>[2x]GFDYDVVVVGGGFAGATAARECGLQGYRTLLLEARSRLGGRTFTSRFAGQEIELGGTWVHWLQPHVWAEMQRYGLGVVEDPLTNLDKTLIMYNDGIVESISPDEFGKNIRIAFEKLCHDAWEVFPRPHEPMFTERARELDKSSVLDRIKTLGLSRLQQAQINSYMALYAGETTDKFGLPGVLKLFACGGWNYDAFMDTETHYRIQGGTIGLINAMLTDSGAEVRMSVPVTAVEQVNGGVKIKTDDDEIITAGVVVMTVPLNTYKHIDFTPALSKGKQRFIKEGQLSKGAKLYVHVKQNLGRVFAFADEQQPLNWVQTRDYSDELGTILSITIARKETIDVNDRDAVTREVQKMFPGVEVLGTAAYDWTADPFSLGAWAAYGVGQLSRLKDLQAAEGRIVFAGAETSNGWHASIDGAVESGLRAGREVKQLLS

Nicotine oxidoreductase (NicA2) is a flavin-dependent enzyme that catalyzes the degradation of nicotine into the non-psychoactive metabolite N-methylmyosmine (NMM). NicA2 acts by degrading nicotine in the bloodstream before it reaches the brain. Clinical use of NicA2 is limited by its poor catalytic activity in the absence of its natural electron acceptor CycN. The higher in vivo activity of NicA2 is due to the presence of a cytochrome c, termed CycN, that acts as an alternative electron acceptor to O29.

We were unable to solve structures of NicA2 v320 but were fortunate to obtain well-diffracting crystals of NicA2 v321 in both the ligand-free and NMM-bound forms. By contrast, the NMM-bound structures of v321 and wild-type NicA2 are very similar with an overall root mean squared deviation of <0.5 Å and no obvious difference that would explain our observed change in activity with O2. Our stopped-flow experiments demonstrated that NicA2 v321 has an increased rate of oxidation compared to the wild-type enzyme, but only when it is bound by the reaction product NMM. The observed increase in the oxidation rate of NMM-bound NicA2 v321 raises an intriguing possibility that the mutations in this variant alter the transport pathway of O2. After addition of NMM to NicA2 v321, we observed a substantial downfield chemical shift in the major peak of the enzyme, possibly due to conformational rearrangement in the tunnel region. We confirmed that these conformational changes are relevant to catalysis by observing a similar spectrum after the addition of nicotine to the enzyme to achieve the NMM-bound, reduced enzyme state that was rapidly oxidized by O2 in our kinetic experiments. Therefore, observations made using the NMM-bound oxidized enzyme report on the conformation of the enzyme relevant for the oxidation step. After NMM binding, NicA2 v321 undergoes major rearrangements in the tunnel region, as indicated by the collapse and substantial downfield shift of fluorine resonances in our 19F experiments. We further demonstrate that this new conformational state is overall more solvent accessible in NicA2 v321 than in wild-type NicA2. This may indicate that the mutations encoded in NicA2 v321 allow greater diffusion of O2 to flavin in this catalytically competent state.>[7x]MEQTQKLKLNLQHFASNNVKPQVFNPDNVMMHEKKDGTLMNEFTTPILQEVMENSKIMQLGKYEPMEGTEKKFTFWADKPGAYWVGEGQKIETSKATWVNATMRAFKLGVILPVTKEFLNYTYSQFFEEMKPMIAEAFYKKFDEAGILNQGNNPFGKSIAQSIEKTNKVIKGDFTQDNIIDLEALLEDDELEANAFISKTQNRSLLRKIVDPETKERIYDRNSDSLDGLPVVNLKSSNLKRGELITGDFDKLIYGIPQLIEYKIDETAQLSTVKNEDGTPVNLFEQDMVALRATMHVALHIADDKAFAKLVPADKRTDSVPGEV

80α is a typical example of a staphylococcal transducing phage, capable of transferring non-specific chromosomal or plasmid DNA at low frequency. The capsids are assembled from a major capsid protein (CP) as empty precursor procapsids into which the DNA is packaged through the portal by the phage terminase. Many SaPIs, such as SaPI1, redirect the 80α capsid assembly pathway to form capsids that are smaller than the normal phage capsids and that are thus incapable of packaging full-length phage genomes. Here, we report the structures of a mature 80α capsid made from an uncleavable version of CP at 5.2 Å resolution and of a wildtype SaPI1 mature capsid at 8.4 Å resolution.

Reasoning that empty particles would be more amenable to 3D reconstruction, since the lack of internal DNA would reduce the background noise, we chose a sample in which the majority of the capsids had ejected their DNA upon prolonged exposure at 22 °C. The reconstruction reached a final resolution of 5.2 Å by the FSC0.143 criterion. Compared to the procapsid, the mature capsid is larger and more angular and has a thinner shell. No density could be assigned for the N-terminal 30 residues of CP, including the N-terminal 14 residues that are normally cleaved from WT capsids. There are considerable differences between the CP subunit in the mature capsid compared to the procapsid, especially in the N-arm, E-loop, P-loop and part of the spine helix (α3). In the mature capsid (which has no SP), the β-strand folds underneath the E-loop that extends from the adjacent subunits, while α1 is rotated by 81° towards the outside of the capsid relative to its orientation in the procapsid. This is accompanied by a straightening of the spine helix (α3) and major changes in the preceding α2 helix and the P-loop (green in Figure 6D), presenting a concerted rotation of the subunit that leads to a disruption of the α-helical palisade seen in the procapsid. During maturation, the CP subunits are rotated from a perpendicular orientation in which the A domains protrude on the surface of the capsid, to a lateral orientation in which both A- and P-domains lie tangentially in the plane of the shell. This rotation is accompanied by a reorganization of the asymmetric, skewed hexamers to almost perfectly six-fold symmetric hexamers. We hypothesize that this rotation is triggered by the release of the N-arm from SP, thereby coupling the capsid expansion to scaffolding removal.In mammals, the E3 ligase Pirh2 mediates the degradation of aberrant nascent polypeptides by targeting the C-terminal polyalanine degrons (polyAla/C-degrons). The E3 ligase Pirh2 (p53-induced RING-H2 protein), also known as Rchy1 (RING finger and CHY zinc finger domain-containing protein 1), encompasses nine zinc binding sites throughout the full-length protein, with six in the N-terminal domain (NTD or CHY zinc finger), two in the central RING domain and one in the C-terminal domain (CTD). Here, we present the crystal structure of Pirh2 bound to the polyAla/C-degron, which shows that the N-terminal domain and the RING domain of Pirh2 form a narrow groove encapsulating the alanine residues of the polyAla/C-degron. Affinity measurements in vitro and global protein stability assays in cells further demonstrate that Pirh2 recognizes a C-terminal A/S-X-A-A motif for substrate degradation.

To better understand the recognition mode of the Ala6/C-degron by Pirh2, we determined the crystal structure of the Pirh2 NTD + RING domains bound to the Ala6/C-degron by fusion of a linker and a six-Ala peptide at the C-terminus. As expected, the Pirh2 NTD and RING coordinate eight zinc ions, whereby each zinc ion is coordinated by four Cys/His residues. Interestingly, the overall structure of NTD + RING forms a π-shaped conformation, with the polyAla tail inserted parallel to the bottom of the width axis. this binding pocket presents a linear and long (~30 Å) deep groove, with an open and a closed end. Specifically, the methyl groups of Ala-1, Ala-2, Ala-4, and Ala-5 each point toward a closed cavity inside the groove walls, while the methyl groups of Ala-3 and Ala-6 point toward the groove opening. Concretely, the free carboxyl group of Ala-1 is positioned to form two hydrogen bonds with the hydroxyl group of Tyr23 and one salt bridge with Arg41. The backbone amide group of Ala-1 forms a direct hydrogen bond with the backbone carbonyl group of Cys108 coordinating the fourth zinc. The Ala-2 is accommodated in a narrow pocket created by NTD and RING, where a backbone hydrogen bond is formed between the amide group of Ala-2 and the carbonyl oxygen of Ser155, and the side chain of Ile107 establishes a hydrophobic interaction with the methyl group of Ala-2. The backbone carbonyl and amide groups form two direct hydrogen bonds with the guanidine group of Arg109 and the backbone carbonyl group of Cys125, respectively. Structural superposition shows that the E2-binding site is located opposite to the Ala6/C-degron binding surface.

>[2x]GMAATAREDGASGQERGQRGCEHYDRGCLLKAPCCDKLYTCRLCHDNNEDHQLDRFKVKEVQCINCEKIQHAQQTCEECSTLFGEYYCDICHLFDKDKKQYHCENCGICRIGPKEDFFHCLKCNLCLAMNLQGRHKCIENVSRQNCPICLEDIHTSRVVAHVLPCGHLLHRTCYEEMLKEGYRCPLCMHSALGSGSGAAAAAA>[8x]GPGSMADFEGKTALITGGARGMGRSHAVA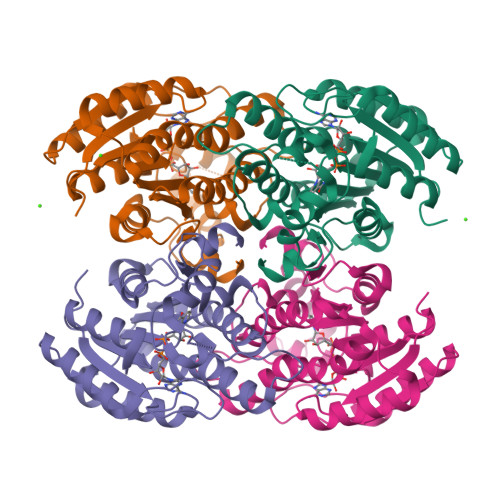LAEAGADIAICDRCENSDVVGYPLATADDLAETVALVEKTGRRCISAKVDVKDRAALESFVAEAEDTLGGIDIAITNAGISTIALLPEVESAQWDEVIGTNLTGTFNTIAAVAPGMIKRNYGRIVTVSSMLGHSANFAQASYVSSKWGVIGLTKCAAHDLVGYGITVNAVAPGNIETPMTHNDFVFGTMRPDLEKPTLKDVESVFASLHLQYAPFLKPEEVTRAVLFLVDEASSHITGTVLPIDAGATARMI> MGLLKDLSSARDKIERIYGLNKEKLLLLAKVKEGFETSVFDFPFKNIQPDSPYFVCLDPPCKKESAYNKVIGDKNRTVYHEINKTEFENMIKLRTKRLKLLIGEVDAEVSTGDKIEFPVLANGKRRGFIYNVGGLVTDIAWLNIEENTDIGKDIQYLAVAVSQYMDEPLNEHL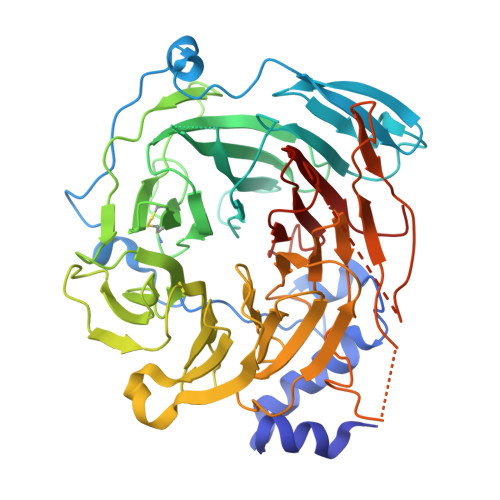EMFDKEKHSSCIQIFKMNTSTLHCVKVQTIVHSFGEVWDLKWHEGCHAPHLVGCLSFVSQEGTINFLEIIDNATDVHVFKMCEKPSLTLSLADSLITTFDFLSPTTVVCGFKNGFVAEFDLTDPEVPSFYDQVHDSYILSVSTAYSDFEDTVVSTVAVDGYFYIFNPKDIATTKTTVSRFRGSNLVPVVYCPQIYSYIYSDGASSLRAVPSRAAFAVHPLVSRETTITAIGVSRLHPMVLAGSADGSLIITNAARRLLHGIKNSSATQKSLRLWKWDYSIKDDKYRIDSSYEVYPLTVNDVSKAKIDAHGINITCTKWNETSAGGKCYAFSNSAGLLTLEYLSLEHHHHHH2-[[(2~{R},3~{S},4~{R},5~{R})-5-(6-aminopurin-9-yl)-3,4-bis(oxidanyl)oxolan-2-yl]methyl-[3-[6-azanyl-9-[(2~{R},3~{R},4~{S},5~{R})-5-[(2-azanylethylcarbamoylamino)methyl]-3,4-bis(oxidanyl)oxolan-2-yl]purin-8-yl]prop-2-ynyl]amino]ethanoic acid | C28 H36 N14 O9 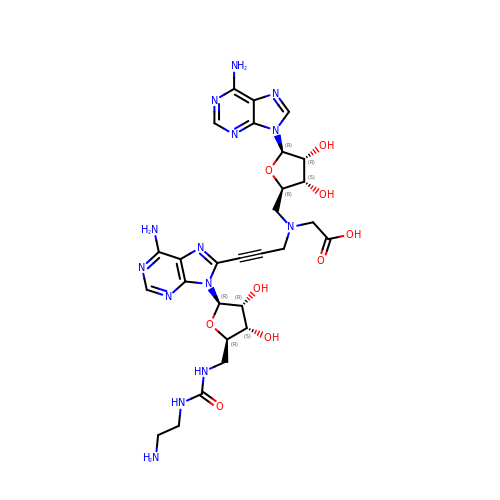| NHZDFSAEZKJJHU-GMIOVBLFSA-N>MTNIVGRIGFLTTGKLGIKLRGVLIDESTTPNTTYLPGIESFFNITANVLTSVSYPETETQNVTATFSIYSVDGSSNPVFPALLSFDAIVPNVASVEFDVLAPTGVVNNQLDTSALRIAKIIANDPALAQKVAGAPYPRGAYSATETYLYGEMVSYFGKNYISKSLSPIINILPTVTDSWYELVITLPESVSVIATGSDTAYGTGWNGSLLVPTQNAVYDKIVTVDAAIATANTNITNLGTAKADLSYVNTQLSADQVVLDALSSGKADLSYVNTQLNSKANLNGAVLVNATTATPPISDNDTSLATTQHVRSFNHSRLAFNAFRGGQQGVPSLSYVTTTAQFNSSSVRSGWGDNFSSNRWLVGEGGTYLITVTTRFATVGGTPPTYFDALLFVGLSGSGVENFLTRSQSVYPSFGYTLSWVGILTFNTGQNVFLNYQVNAVGGGSYSVVLEDVRFSGIQLG[3x]

A-1(L) is a Myoviridae cyanophage isolated in 1970s9 that specifically infects the model cyanobacterium Anabaena sp. PCC 7120. Using cryo-electron microscopy (cryo-EM), we solved the structure of A-1(L) tail machine, which consists of three parts: a 205-Å-long neck, a 1045-Å-long contractile tail with a complicated baseplate, and six pairs of tail fibers. The dodecameric gp2 portal, the pentadecameric gp5 and the hexameric gp7 sequentially constitute the neck of A-1(L), to which five neck fibers are attached. The long and contractile tail of A-1(L) contains 24 rings of gp10 hexamers that form the tube, surrounded by the sheath of 24 helically stacked gp9 hexamers.

Each LTF subunit contains a shoulder and an arm domain, whereas each STF subunit consists of four domains: β-ring, joint, stem and cell wall binding domain (CBD). Structural analysis showed that the arm domain of LTF and the CBD domain of STF most likely possess the binding motifs that recognize the host receptors. Using in vitro binding assays, we observed that the arm domain of LTF, but not the CBD domain of STF, binds to the cell surface of Anabaena sp. PCC 7120. In contrast, the stem-CBD domain of STF could bind to the host cell surface. Further competition binding assays showed that the arm domain of LTF and the stem-CBD domain of STF could simultaneously bind to the surface of host cells. Altogether, it suggested that the STF/gp33 and LTF/gp34 are indeed RBPs, which recognize and bind to different receptors on the host cell surface. For A-1(L), we previously found that antibodies against either STF or LTF could strongly inhibit the infection, suggesting that they might be essential for the adsorption of A-1(L) to the host cell surface.> MRGMLPLFEPKGRVLLVDGHHLAYRTFHALKGLTTSRGEPVQAVYGFAKSLLKALKEDGDAVIVVFDAKAPSFRHEAYGGYKAGRAPTPEDFPRQLALIKELVDLLGLARLEVPGYEADDVLASLAKKAEKEGYEVRILTADKDLYQLLSDRIHVLHPEGYLITPAWLWEKYGLRPDQWADYRALTGDESDNLPGVKGIGEKTARKLLEEWGSLEALLKNLDRLKPAIREKILAHMDDLKLSWDLAKVRTDLPLEVDFAKRREPDRERLRAFLERLEFGSLLHEFGLLESPKALEEAPWPPPEGAFVGFVLSRKEPMWADLLALAAARGGRVHRAPEPYKALRDLKEARGLLAKDLSVLALREGLGLPPGDDPMLLAYLLDPSNTTPEGVARRYGGEWTEEAGERAALSERLFANLWGRLEGEERLLWLYREVERPLSAVLAHMEATGVRLDVAYLRALSLEVAEEIARLEAEVFRLAGHPFNLNSRDQLERVLFDELGL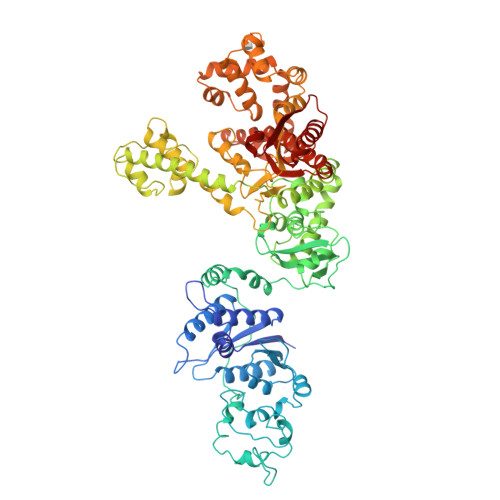PAIGKTEKTGKRSTSAAVLEALREAHPIVEKILQYRELTKLKSTYIDPLPDLIHPRTGRLHTRFNQTATATGRLCCCDPNLQNIPVRTPLGQRIRRGFIAEEGWLLVALDYSQIELRVLAHLSGDENLIRVFQEGRDIHTETASWMFGVPREAVDPLMRRAAKTINFGVLYGMSAHRLSQELAIPYEEAQAFIERYFQSFPKVRAWIEKTLEEGRRRGYVETLFGRRRYVPDLEARVKSVREAAERMAFNMPVQGTAADLMKLAMVKLFPRLEEMGARMLLQVHDELVLEAPKERAEAVARLAKEVMEGVYPLAVPLEVEVGIGEDWLSAKE>[2x]MKHTGLFKTLCFCAGCLLLSACVDYSDIQPFDGKTLPRKSGYTTGVTNDWIYFNLRTGEIFNALGVNRDIKEGGQMNRTDWDLAFCGYVMRTNSGTSGIGRGGAADLGYGNYEN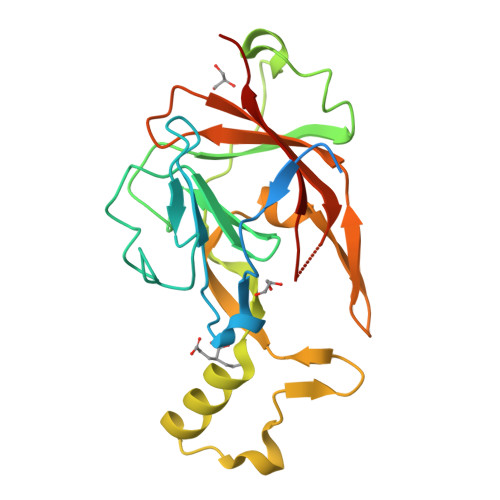WTSVAQLPSDLKWVEDNQEVYVTMSQNDWNHYLIENGLDFNSNPWFDPNNGPQKTTTNANPVLAQAMSFAGPPPVYTPSYHTYVVRTADGKHYFKIQIISWYDANVEIGDEGGRLSYYCDELQP2-(4-AMINOBENZYL)-1,3-DIOXO-2,3-DIHYDRO-1H-BENZO[DE]ISOQUINOLINE-5-SULFONATE | C19 H13 N2 O5 S | 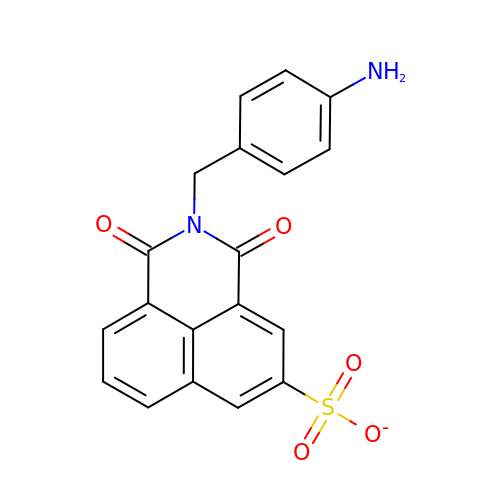DTGCLOCEXRIHBE-UHFFFAOYSA-M> WSHPQFEKVPIKYLPEENVHDADFGEQKDISEINLAAGLDLFQGDILLQKSRNGLRDPNTRWTFPIPYILADNLGLNAKGAILYAFEMFRLKSCVDFKPYEGESSYIIFQQFDGCWSEVGDQHVGQN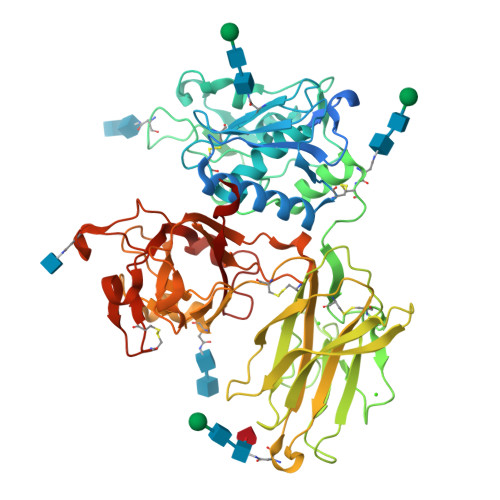ISIGQGCAYKAIIEHEILHALGFYHEQSRTDRDDYVNIWWDQILSGYQHNFDTYDDSLITDLNTPYDYESLMHYQPFSFNKNASVPTITAKIPEFNSIIGQRLDFSAIDLERLNRMYNCTTTHTLLDHCTFEKANICGMIQGTRDDTDWAHQDSAQAGEVDHTLLGQCTGAGYFMQFSTSSGSAEEAALLESRILYPKRKQQCLQFFYKMTGSPSDRLVVWVRRDDSTGNVRKLVKVQTFQGDDDHNWKIAHVVLKEEQKFRYLFQGTKGDPQNSTGGIYLDDITLTETPCPTGVWTVRNFSQVLENTSKGDKLQSPRFYNSEGYGFGVTLYPNSRESSGYLRLAFHVCSGENDAILEWPVENRQVIITILDQEPDVRNRMSSSMVFTTSKSHTSPAINDTVIWDRPSRVGTYHTDCNCFRSIDLGWSGFISHQMLKRRSFLKNDDLIIFVDFEDITHLS>GHMGITAIALYDYQAAGDD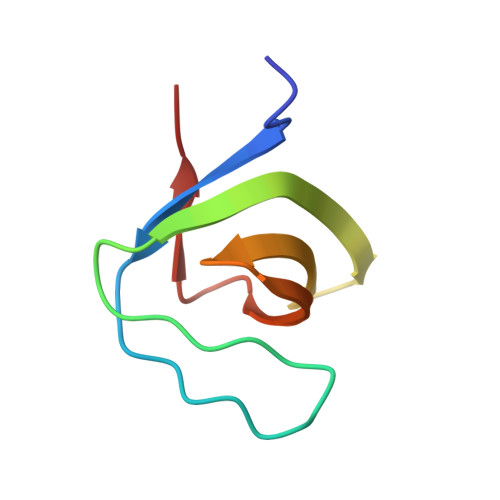EISFDPDDIITNIEMIDDGWWRGVCKGRYGLFPANYVELRQ[6x]>[5x]ALSKVKLNDTLNKDQLLSSSKYTIQRSTGDSIDTPNYDVQKHINKLCGMLLITEDANHKFTGLIGMLYAMSRLGREDTIKILRDAGYHVKANGVDVTTHRQDINGKEMKFEVLTLASLTTEIQINIEIESRKSYKKMLKEMGEVAPEYRHDSPDCGMIILCIAALVITKLAAGDRSGLTAVIRRANNVLKNEMKRYKGLLPK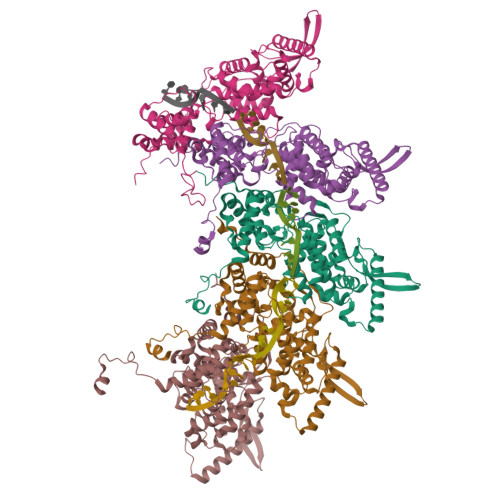DIANSFYEVFEKHPHFIDVFVHFGIAQSSTRGGSRVEGIFAGLFMNAYGAGQVMLRWGVLAKSVKNIMLGHASVQAEMEQVVEVYEYAQKLGGEAGFYHILNNPKASLLSLTQFPHFSSVVLGNAAGLGIMGEYRGTPRNQDLYDAAKAYAEQLKENGVINYSVLDLTAEELEAIK benzenethiol 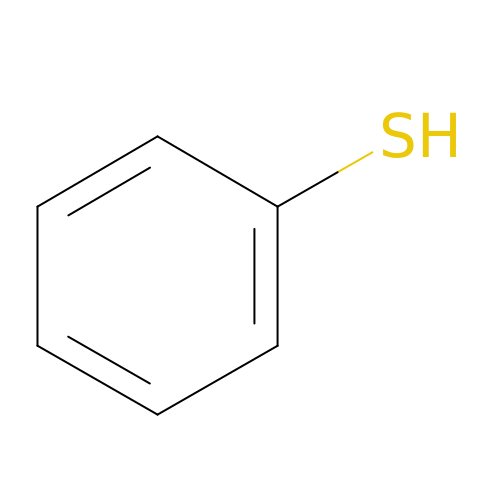| C6 H6 S | RMVRSNDYEFQCLF-UHFFFAOYSA-N>[2x]MARTGALLLVALALAGCAQACIYK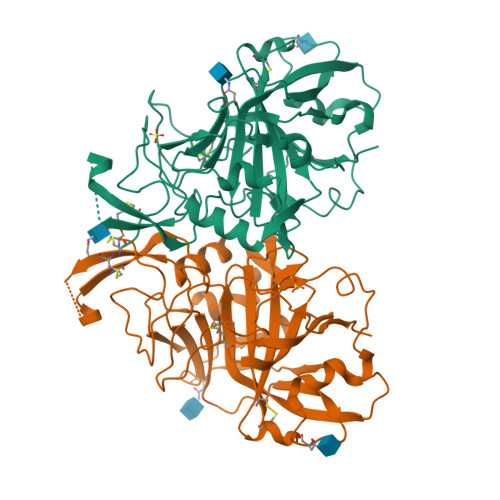FGTSPDSKATVSGDHWDHGLNGENWEGKDGAGNAWVCKTGRKQSPINVPQYQVLDGKGSKIANGLQTQWSYPDLMSNGTSVQVINNGHTIQVQWTYNYAGHATIAIPAMHNQTNRIVDVLEMRPNDAADRVTAVPTQFHFHSTSEHLLAGKIYPLELHIVHQVTEKLEACKGGCFSVTGILFQLDNGPDNELLEPIFANMPSREGTFSNLPAGTTIKLGELLPSDRDYVTYEGSLTTPPCSEGLLWHVMTQPQRISFGQWNRYRLAVGLKECNSTETAADAGHHHHHRRLLHNHAHLEEVPAATSEPKHYFRRVMLAESANPDAYTCKAVAFGQNFRNPQYANGRTIKLARYH Toxoplasma gondii is one of the most significant parasites that impacts human health, with estimates that as many as one third to one half of the human population are infected. At the Center for Structural Genomics of Infectious Diseases (CSGID), the first Toxoplasma Structural Genomics Pipeline was established. The enzymes selected from the TDR database as small and tractable for expression and crystallization included: phosphoglycerate mutase II (hereafter referred to as PGM), nucleotide diphosphate kinase (NDK), ribulose phosphate 3-epimerase (RPE), ribose-5-phosphate isomerase (RPI), and ornithine aminotransferase (OAT). The genes encoding these enzymes were cloned, proteins expressed and purified, crystallized, and crystal structures were determined.

Ribulose phosphate 3-epimerase functions in the conversion of ribulose-5-phosphate into xylulose-5-phosphate, which is a reaction in the Calvin cycle. TgRPE adopts an aldolase-type TIM-barrel α/β fold resembling homologous RPEs. Four chains of TgRPE (~0.3–0.5 Å r.m.s.d. over 225 Cα atoms) in the H32 asymmetric unit form two dimers each burying a surface area of ~3,500 Å2. Helices α1 and α2, and the β2–α2 and η1– α1 loops of TgRPE comprise the dimer interface with 4 salt bridges, 8 hydrogen-bonded and 130 van der Waals contacts (e.g., between chains A and C). PISA prediction and crystal packing analysis revealed a hexameric assembly of TgRPE (BSA is ~13,300 Å2; not shown) that has been reported previously for homologous RPEs. A Zn2+ (e.g., ZN 303/A) ion was modeled per each chain of TgRPE, with His37, Asp39, His71, Asp182 and a water molecule coordinating the metal. The CheckMyMetal analysis identified that Co2+ and Cu2+ may also bind in a similar position as zinc in TgRPE. Crystals of TgRPE grew in the presence of 500 mM NaCl and 2 M ammonium sulfate and, thus multiple sulfate and chloride ions were modeled to interpret additional electron density. In addition, the presence of SO42- in the active site induces the β6–α5 loop to move from its presumed apo conformation in the absence of ligand, as seen in the human RPE homolog, to holo conformation in the ligand bound state. Additional experiments are needed to confirm the biological importance of zinc in the TgRPE-based catalysis.

>[4x]MSSQLKPIICPSVLASDLSSLASDAKRMVDAGCDWLHLDIMDGHFVPNISFGPGVVKALRGHLKSAFFDVHLMVSEPEKWIQPFADAGANSITFHWESVGGDLQRAAELAKRIQARGIKAGLAIKPATKFEDLGEALAGDNFDMLLVMTVEPGFGGQKFMADMLQKVRTARSLFPKLNIQVDGGLDGETVKPAASAGANVIVAGTSMFKAENPAALMTFMRDVIAASDTLGENLYFQSAGHHHHHH> GMRCNERNKKKAIFSNDDFSGEDTLMEDHLQLREKLSEDIEMIKASLKNNLVCSTLNDNEILTLSNYMQFFVFKGGDLVIKQGEKGSYFFIINSGKFDVYVNDKKVKSMGKGSSFGEAALIHNTQRSATIMAETDGTLWGVQRSTFRATLKQLSNRNFNENRSFIDSVSVFDMLTEAQKNMITNACVIQMFKPGETIVKQGDYGDVLFILKEGKATVFINDKEIRVLNKGSYFGERALLYDEPRSATIIAKEPTACASICRKLLNIVLGNLQVVLFRNIMTEALQQSEIFRQFSAEQLNDLADTAIVRDYPANYHILHKDKVKSVKYLIVLEGKVELFLDDESIGILTRGKSFGDQYVLNQKQKFRHTVKSLDVCKIALITESCLADCLGDNNIDASIDHNNKKSIIKKMYIFRYLSEQQ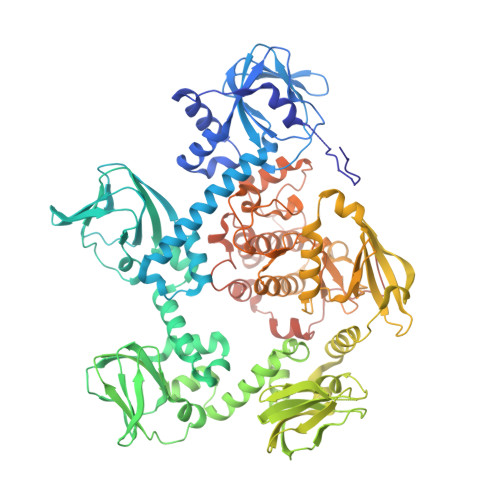CNLLIEAFRTTRYEEGDYIIQEGEVGSRFYIIKNGEVEVTKNGKRLRTLGKNDYFGERALLYDEPRTASIISKATSVECWFVDKSVFLQIIQGPMLTHLEERIKMQDTKVEMHELETERIIGRGTFGTVKLVHHKPTQIRYALKCVSKRSIISLNQQNNIKLEREITAENDHPFIIRLVRTFKDSNCFYFLTELVTGGELYDAIRKLGLLSKPQAQFYLGSIILAIEYLHERNIVYRDLKPENILLDKQGYVKLIDFGCAKKIQGRAYTLVGTPHYMAPEVILGKGYGCTVDIWALGVCLYEFICGPLPFGNDQEDQLEIFRDILTGQLTFPDYVSDQDSINLMKRLLCRLPQGRIGCSINGFKDIKEHAFFGNFNWDKLAGRLLEPPLVSKGETYAEDIDIKQIEEEDALNEGEPLDGDDSWDVDF>MGTEPPENCQDDFNFNYVSDQEIEVYHVDKGWSAGWNYVCLNDYCLPGNKSNGAFRKTFNAVLGQDYKLTFKVEDRYGQGQQILDRNITFTTQVC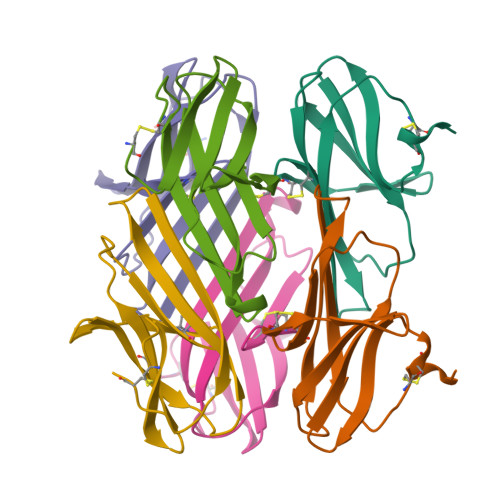NLEHHHHHH[6x]>[2x]GGNSFVGLRVVAKWSSNGYFYSGKITRDVGAGKYKLLFD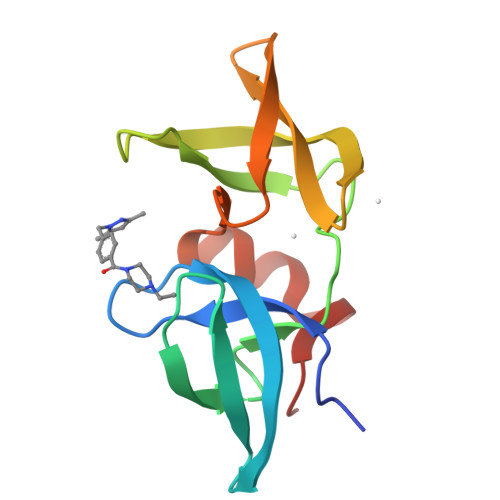DGYECDVLGKDILLCDPIPLDTEVTALSEDEYFSAGVVKGHRKESGELYYSIEKEGQRKWYKRMAVILSLEQGNRLREQYGLGPYE> PNFAGTWKMRSSENFDELLKALGVNAMLRKVAVAAASK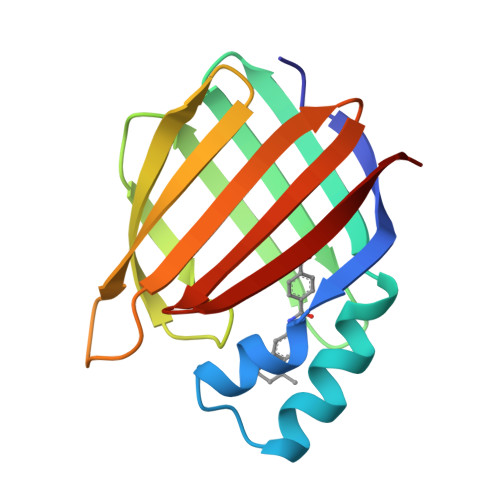PHVEIRQDGDQFYIKTSTTVRTTEINFKVGEGFEEETVDGRKCRSLPTWENENKIHCTQTLLEGDGPKTYWTRELANDELILTFGADDVVCTRIYVRE>MWKVSERCLKGHGKFQADQEIGNGLATAKGQCKGTDSDQKKAGKCDKHCTGVCLGSG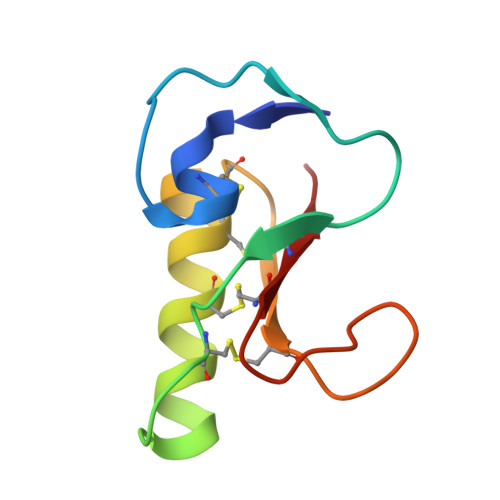GSCGDGSSQKPNKEDCYCKSK[2x]>MTGMSREEVESLIQEVLEVYPEKARKDRNKHLAVNDPAVTQSKKCIISNKKSQPGLMTIRGCAYAGSKGVVWGPIKDMIHISHGPVGCGQYSRAGRRNYYIGTTGVNAFVTMNFTSDFQEKDIVFGGDKKLAKLIDEVETLFPLNKGISVQSECPIGLIGDDIESVSKVKGAELSKTIVPVRCEGFRGVSQSLGHHIANDAVRDWVLGKRDEDTTFASTPYDVAIIGDYNIGGDAWSSRILLEEMGLRCVAQWSGDGSISEIELTPKVKLNLVHCYRSMNYISRHMEEKYGIPWMEYNFFGPTKTIESLRAIAAKFDESIQKKCEEVIAKYKPEWEAVVAKYRPRLEGKRVMLYIGGLRPRHVIGAYEDLGMEVVGTGYEFAHNDDYDRTMKEMGDSTLLYDDVTGYEFEEFVKRIKPDLIGSGIKEKFIFQKMGIPFREMHSWDYSGPYHGFDGFAIFARDMDMTLNNPCWKKLQAPWE[2x];>[2x]SQQVDKIKASYPLFLDQDYKDMLAKKRDGFEEKYPQDKIDEVFQW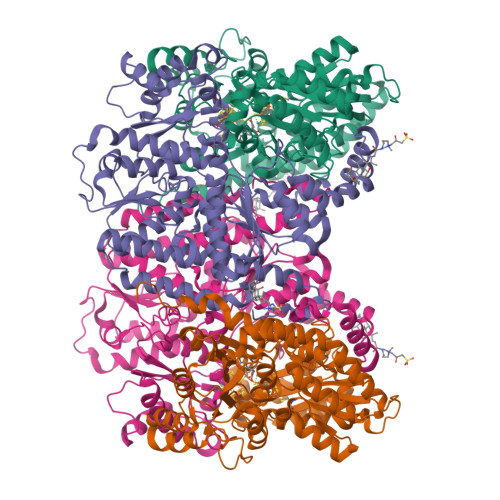TTTKEYQELNFQREALTVNPAKACQPLGAVLCALGFEKTMPYVHGSQGCVAYFRSYFNRHFREPVSCVSDSMTEDAAVFGGQQNMKDGLQNCKATYKPDMIAVSTTCMAEVIGDDLNAFINNSKKEGFIPDEFPVPFAHTPSFVGSHVTGWDNMFEGIARYFTLKSMDDKVVGSNKKINIVPGFETYLGNFRVIKRMLSEMGVGYSLLSDPEEVLDTPADGQFRMYAGGTTQEEMKDAPNALNTVLLQPWHLEKTKKFVEGTWKHEVPKLNIPMGLDWTDEFLMKVSEISGQPIPASLTKERGRLVDMMTDSHTWLHGKRFALWGDPDFVMGLVKFLLELGCEPVHILCHNGNKRWKKAVDAILAASPYGKNATVYIGKDLWHLRSLVFTDKPDFMIGNSYGKFIQRDTLHKGKEFEVPLIRIGFPIFDRHHLHRSTTLGYEGAMQILTTLVNSILERLDEETRGMQATDYNHDLVR>[2x]MVGLEDDTERERSPVVENGFSNGSRSSSSSAGVLSPSRKVTQGNDTLSYANILRARNKFADALALYEAMLEKDSKNVEAHIGKGICLQTQNKGNLAFDCFSEAIRLDPHNACALTHCGILHKEEGRLVEAAESYQKALMADASYKPAAECLAIVLTDLGTSLKLAGNTQEGIQKYYEALKIDPHYAPAYYNLGVVYSEMMQYDNALSCYEKAALERPMYAEAYCNMGVIYKNRG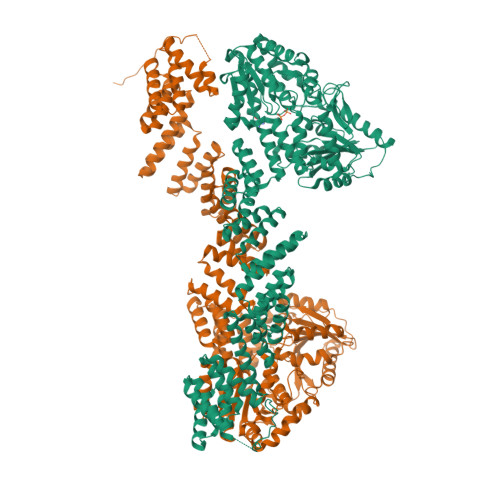DLEMAITCYERCLAVSPNFEIAKNNMAIALTDLGTKVKLEGDVTQGVAYYKKALYYNWHYADAMYNLGVAYGEMLKFDMAIVFYELAFHFNPHCAEACNNLGVLYKDRDNLDKAVECYQMALSIKPNFAQSLNNLGVVYTVQGKMDAAASMIEKAILANPTYAEAFNNLGVLYRDAGNITMAIDAYEECLKIDPDSRNAGQNRLLAMNYINEGLDDKLFEAHRDWGWRFTRLHPQYTSWDNLKDPERPITIGYISPDFFTHSVSYFIEAPLTHHDYTKYKVVVYSAVVKADAKTYRFRDKVLKKGGVWKDIYGIDEKKIASMVREDKIDILVELTGHTANNKLGTMACRPAPVQVTWIGYPNTTGLPTVDYRITDSLADPPDTKQKQVEELVRLPDCFLCYTPSPEAGPVSPTPALSNGFVTFGSFNNLAKITPKVLQVWARILCAVPNSRLVVKCKPFCCDSIRQRFLTTLEQLGLESKRVDLLPLILFNHDHMQAYSLMDISLDTFPYAGTTTTCESLYMGVPCVTMAGSVHAHNVGVSLLTKVGLGHLVAKNEDEYVQLSVDLASDVTALSKLRMSLRDLMAGSPVCNGPSFAVGLESAYRNMWKKYCKGEVPSLRRMEMLQKEVHDDPLISKDLGPSRVSVTGEATPSLKANGSAPVPSSLPTQSPQLSKRMDSTS>MSSAQRVVITPGEPAGSGPDLVVQLAQRAWPIELVVCADGALLTERAAMLGLPLSLLPYSPDVPAAPQPAGTLTLLPVSLRAPAISGQLTVENGPYVVETLARACDGCLNGEFAA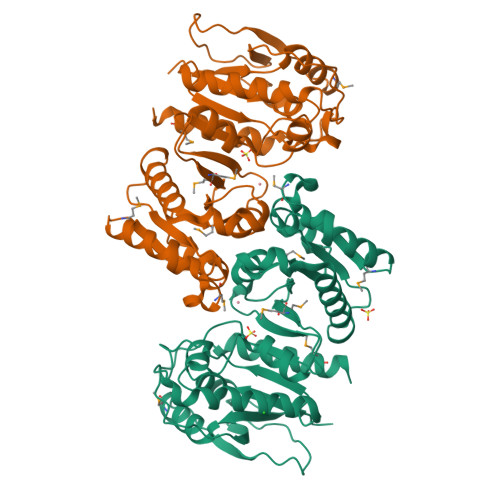LITGPVHKGVINDAGISFTGHTEFFEERSQAKKVVMMLATEELRVALATTHLPLRAIADAITPALLHEVIAILHHDLRTKFGIAEPRILVCGLNPHAGEGGHMGTEEIDTIIPVLDELRAQGMKLNGPLPADTLFQPKYLDNADAVLAMYHDQGLPVLKYQGFGRGVNITLGLPFIRTSVDHGTALELAGRGKADVGSFITALNLAIKMIVNTQ[2x]Polymerases generate nascent strands of genetic material by stepwise phosphoryl transfer of nucleotides to primer termini, yielding O3′→P5′ phosphodiester linkages. We reported that 3′-NH2 primer extension can be catalyzed by a modified DNA polymerase, yielding N3′→P5′ phosphoramidate DNA (NP-DNA). The large fragment of DNA polymerase I (BF), cloned from the thermophilic soil bacterium Geobacillus stearothermophilus (Bst), acquires nontrivial levels of N3′→P5′ polymerase activity via two surprisingly minor substitutions: (A) a single active site mutation (F710Y) and (B) substitution of its divalent Mg2+ cofactors with Ca2+ (1). To add evidence that a single divalent metal ion cofactor catalyzes unnatural NP synthesis in BF, a polymerase A family member, we carried out a single nucleotide primer extension reaction in intact crystals.

We crystallized active substrate-bound BF polymerase F710Y/D598A with a 3′-amino terminal DNA primer and DNA template in the presence of Ca2+ and 2′-deoxyguanosine 5′-triphosphate (dGTP). Reactions were then initiated in the intact crystals by pH-shift from an acidic mother liquor (pH < 6) to a basic soaking liquor at pH 8.8, and reacting crystals were quenched at various times by flash freezing. Early time points show negligible differences in ordered density between the ground state complex crystallized under acidic conditions versus the complex after 1 h of soaking under reaction conditions, suggesting that the reactant state and ground state cannot be clearly distinguished in this resolution range. The conserved Asp-830 side chain, proximal to the nucleophilic primer 3′-amine at ~2.5 Å in refined ground state structures, is the most likely general base mediating this proton transfer. The lack of electron density for an A-site metal ion in the ground state and at later time points is also consistent with the expectation of a neutral nucleophile in the NP reaction and the generally weak affinity of aliphatic amines for Ca2+. Unlike for native phosphodiester catalysis, only a single metal ion cofactor is detectable by crystallography during NP catalysis.

>[2x]KMAFTLADRVTEEMLADKAALVVEVVEENYHDAPIVGIAVVNEHGRFFLRPETALADPQFVAWLGDETKKKSMFDSKRAAVALKWKGIELCGVSFDLLLAAYLLDPAQGVDDVAAAAKMKQYEAVRPDEAVYGKGAKRAVPDEPVLAEHLVRKAAAIWELERPFLDELRRNEQDRLLVELEQPLSSILAEMEFAGVKVDTKRLEQMGKELAEQLGTVEQRIYELAGQEFNINSPKQLGVILFEKLQLPVLKKTKTGYSTSADVLEKLAPYHEIVENILHYRQLGKLQSTYIEGLLKVVRPATKKVHTIFNQALTQTGRLSSTEPNLQNIPIRLEEGRKIRQAFVPSESDWLIFAADYSQIELRVLAHIAEDDNLMEAFRRDLDIHTKTAMDIFQVSEDEVTPNMRRQAKAVNYGIVYGISDYGLAQNLNISRKEAAEFIERYFESFPGVKRYMENIVQEAKQKGYVTTLLHRRRYLPDITSRNFNVRSFAERMAMNTPIQGSAADIIKKAMIDLNARLKEERLQAHLLLQVHDELILEAPKEEMERLCRLVPEVMEQAVTLRVPLKVDYHYGSTWYDAK>[4x]MTPNIYQQLGLKKVINACGKMTILGVSSVAPEVMQATARAASAFVEIDALVEKTGELVSRYTGAEDSYITSCASAGIAIAVAAAITHGDRARVALMPDSSGMANEVVMLRGHNVDYGAPVTSAIRLGGGRIVEVGSSNLATRWQLESAINEKTAALLYVKSHHCVQKGMLSIDDFVQVAQANHLPLIVDAAA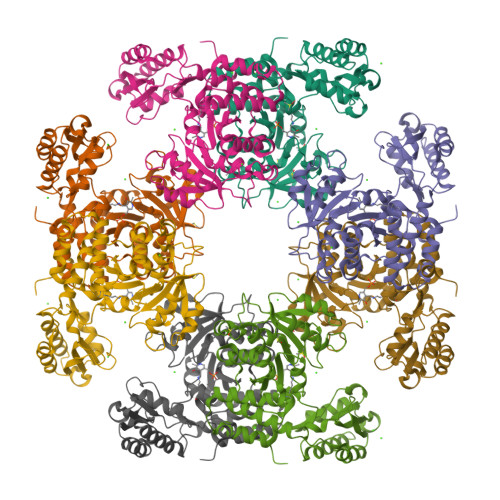EEDLRGWVASGADMVIYSGAKAFNAPTSGFITGRKTWIAACKAQHQGIARAMKIGKENMVGLVYALENYHQGQTTVTAAQLQPVAEAISAIHGLYADIEQDEAGRAIWRIRVRVNASELGLNAQDVEAQLRGGEIAIYARKYQLHQGVFSLDPRTVAEGEMALIVARLREIAEHAAD>GPHMLEREKIYQWINELSSPETRENALLELSKKRESVPDLAPMLWHSFGTIAALLQEIVNIYPSINPPTLTAHQSNRVCNALALLQCVASHPETRSAFLAAHIPLFLYPFLHTVSKTRPFEYLRLTSLGVIGALVKTDEQEVINFLLTTEIIPLCLRIMESGSELSKTVATFILQKILL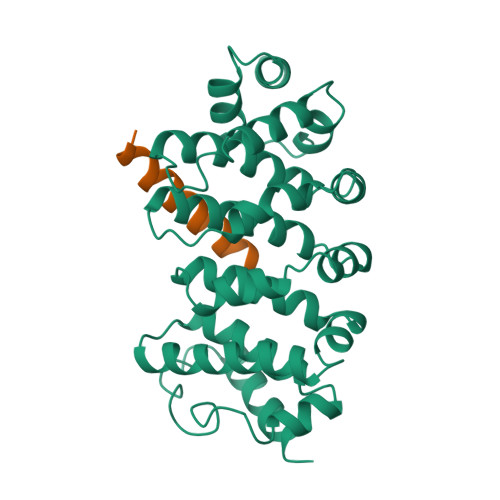DDTGLAYICQTYERFSHVAMILGKMVLQLSKEPSARLLKHVVRCYLRLSDNPRAREALRQCLPDQLKDTTFAQVLKDDTTTKRWLAQLVKNLQE[4x];>[4x]DDQQLDHNFKQMEEHLALMVEGNE>VEKNITVTASVDPAIDLLQADGNALPSAVKLAYSPASKTFESYRVMTQVHTNDATKKVIVKLADTPQLTDVLNSTVQMPISVSWGGQVLSTTAKEFEAAALGYSASGVNGVSSSQELVISAAPKTAGTAPTAGNYSGVVSLVMTLG[13x]

To attach to intestinal cells ETEC express colonization factors, among them CFA/I, which are the most prevalent factors and are the archetypical representative of class 5 pili. The bioassembly of CFA/I pili is initiated by the attachment of the chaperone/minor pilin (CfaA/CfaE) heterodimer to the usher protein CfaC at the outer membrane assembly site followed by cyclic incorporation of the major pilin, CfaB. Adhesion pili subunits are assembled into helical polymers after being chaperoned across the periplasm, transported through an usher protein that resides in the outer membrane, and pilins are then sequentially added to the growing pilus filament. This pilus assembly occurs via a ‘donor-strand exchange’ during which the N-terminal extension (NTE) of each pilin subunit is transferred from the chaperone protein to a growing chain of pilin subunits, filling an empty groove in the previous subunit. The helical quaternary structure of CFA/I can be unwound under tensile force and it has been shown that this mechanical property helps bacteria to withstand shear forces from fluid motion.

We report in this work the CFA/I pilus structure at 4.3 Å resolution from electron cryomicroscopy (cryo-EM) data, and report details of the donor strand complementation. After rigid-body fitting of the subunit’s structure determined by X-ray crystallography into the cryo-EM helical reconstruction, we used RosettaCM to refine the filament structure of CfaB based upon the cryo-EM map. CFA/I pili are assembled using the NTE of subunit n fitted into the groove created by a ‘missing β-strand’ in the previously added subunit, n − 1. Calculated from our CFA/I model using CocoMaps software the buried surface area between subunits n and n + 3 is 1087 Å2, whereas the buried surface area between n and n + 1 is 485 Å2, and between n and n + 2 is 453 Å2. Our findings suggest that quaternary structural stability for CFA/I pili is due mainly to the stacking interface formed by every n to n + 3 contact, as demonstrated by this contact having the largest buried surface area, 1087 Å2. In the current structure, Pro13 has a better fit in a trans conformation, in contrast to the expectation that a transition from trans to cis would produce the rotation required for the conformational change from a linear to a helical structure. While at our current resolution, an unambiguous fit of Pro13 into the EM map is not possible, bending of the backbone structure between Pro13 and Ala14 appears to provide the rotation necessary for assembly of the helical filament.> SNKKTKLIHGGHTTDDYTGAVTTPIYQTSTYLQDDIGDLRQGYEYSRTANPTRSSVESVIATLENGKHGFAFSSGVAAISAVVMLLDKGDHIILNSDVYGGTARALTKVFTRFGIEVDFVDTTHTDSIVQAIRPTTKMLFIETPSNPLLRVTDIKKSAEIAKEHGLISVVDNTFMTPYYQNPLDLGIDIVL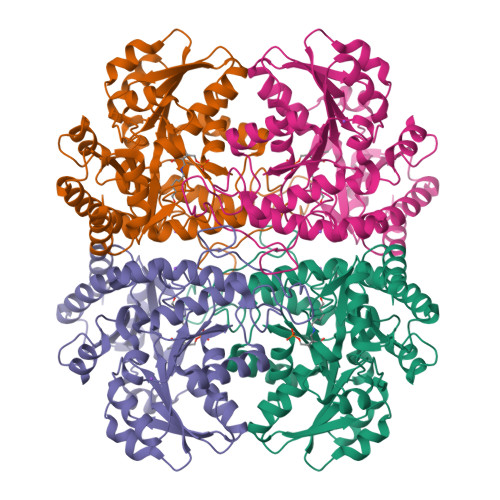HSATKYLGGHSDVVAGLVATSDDKLAERLAFISNSTGGILGPQDSYLLVRGIKTLGLRMEQINRSVIEIIKMLQAHPAVQQVFHPSIESHLNHDVHMAQADGHTGVIAFEVKNTESAKQLIKATSYYTLAESLGAVESLISVPALMTHASIPADIRAKEGITDGLVRISVGIEDTEDLVDDLKQALDTL>TRRTAFFFDELCLWHAAGPHALTLPVGGWVQPPAAAGHAESPETKRRLKSLLDVSGLTARLQLRSAPPASDEDLLRVHPAHYLERFKALSDAGGGSLGQDAPIGPGSYEIARLSAGLAIAALDAVLAGEADNAYSLSRPPGHHCLPDQAMGFCFFANIAVAIEAAKARHGVERVAVLDWDVHHGNGTQAIYYRRDDVLSISLHQDGCFPPGYSGAEDIGEDRGRGFNLNVPLLPGGGHDAYMQAMQRIVLPALERFRPQLIVVASGFDANAVDPLARMQLHSDSFRAMTAMVRDAAERHAG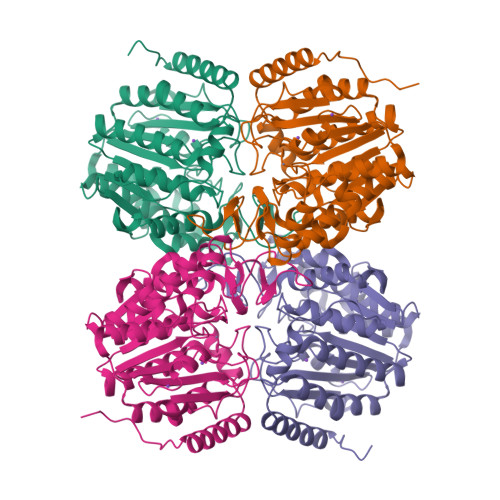GRLVVVHEGGYSEAYVPFCGLAVIEELSGVRSAVRDPLRDFIELQQPNAAFRDFQRQRLEELAAQFGLCPAQPLQAAR[2x]>MASTATVATTPEGIPVIILKEGSSRTYGKEAVRANIAAVKAVEEALKSTYGPRGMDKMLVDSLGDITITNDGATILDKMDLQHPAAKLLVQIAKGQDEETADGTKTAVIFSGELVKKAEDLLYKDVHPTIIISGYKKAEEVALQTIQELAQTVSINDTDLLRKIAMTSLSSKAVAGAREYIADIVVKAVTQVAELRGDKWYVDLDNIQIVKKAGGSINDTQLVYGIVVDKEVVHPGMPKRLENAKIALIDASLEVEKPELDAEIRINDPTQMQKFLDEEENLIKEKVDKILATGANVIICQKGIDEVAQSYLAKKGVLAVRRAKKSDLEKLARATGGRVVSNIDEISEQDLGYASLIEERKVGEDKMVFVEGAKNPKSISILIRGGLERLVDETERALRDALGTVADVIKDGRAIAGGGAVEIEIAKKLRKYAPQVGGKEQLAVEAYANALESLVSILIENAGFDPIDLLMKLRSTHENENNKWYGIDLYAGQPVDMWQKGVIEPALVKMNAIKAATEAATLVLRIDDVVSAGKKSGGESKTPGGANKPSEED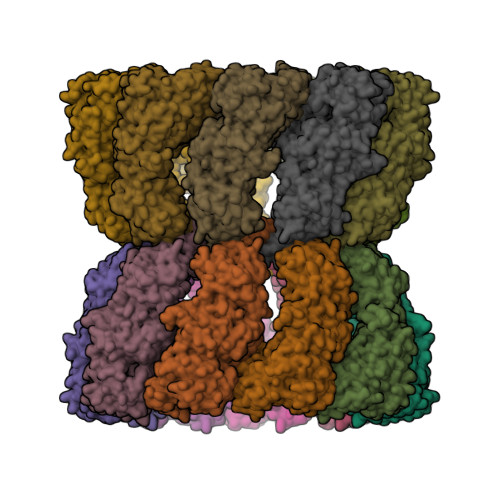[9x]>GPGVPSMAAITSIMRAQQILLGEVDAVVKPYGLTFARYEALVLLTFSKSGELPMSKIGERLMVHPTSVTNTVDRLVRSGLVAKRPNPNDGRGTLATITDKGREVVEAATRDLM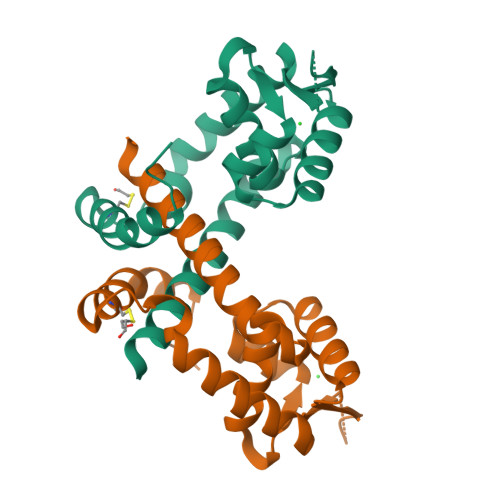AMDFGLGAYDAEECGEIFAMLRPLRVAAGDFDED[2x]>[5x]MLVSVYLALLVACVGQAHSQANLMRLKSDLFNRSPMYPGPTKDDPLTVTLGFTLQDIVKVDSSTNEVDLVYYEQQRWKLNSLMWDPNEYGNITDFRTSAADIWTPDITAYSSTRPVQVLSPQIAVVTHDGSVMFIPAQRLSFMCDPTGVDSEEGVTCAVKFGSWVYSGFEIDLKTDTDQVDLSSYYASSKYEILSATQTRQVQHYSCCPEPYIDVNLVVKFRERRAGNGFFRNLFDENLYFQGHHHHHH

Protein-engineering methods have been exploited to produce a surrogate system for the extracellular neurotransmitter-binding site of a heteromeric human ligand-gated ion channel, the glycine receptor. Acetylcholine-binding protein is a highly conserved ortholog of the pLGIC extracellular ligand-binding domain (ECD) with properties similar to nAChR. Mutations affecting key residues in the orthosteric agonist site at the α1(−)/β(+) interface affect the potency of both activation by glycine and inhibition by strychnine. We therefore set out to generate a high-fidelity surrogate of this α1(−)/β(+) orthosteric binding site using the 2α1:3β stoich­iometry [Fig. 1(a)] by exploiting protein-engineering methods and the thermal stability of acetylcholine-binding protein from Aplysia californica (AcAChBP). Ultimately, the highly stable AcAChBP framework has allowed us to introduce nine amino-acid substitutions that have resulted in a stable surrogate for a heteromeric neurotransmitter site that binds glycine.

A previously published structure of the WT AcAChBP–strychnine complex shows a single molecule occupying four of the five orthosteric sites in the asymmetric unit and one site with two ligands bound. We note also that this alkaloid displays a propensity to dimerize or aggregate at high concentrations. Our structure of the WT AcAChBP–strychnine complex displays a single well ordered strychnine in all five binding sites per asymmetric unit and we confine our comparison to this binding pose. The orientation and the position of the alkaloid in both WT AcAChBP structures is very similar. There is a single direct hydrogen bond between the alkaloid and the protein donated by the protonated tertiary amine to the carbonyl of Trp164. The potential hydrogen-bond acceptors on strychnine, ether and amide O atoms, are placed to interact with solvent and in so doing then form bridges to the protein. Strychnine is a promiscuous ligand that is active against different receptors. Electrophysiological assays indicate that the alkaloid, although the prototypical competitive antagonist of GlyR, also displays the same activity against some nAChR subtypes, with IC50 values that range from 350 nM to around 40 µM. The affinity of strychnine interacting with AcAChBP is consistent with the activity that this ligand displays against the orthologous binding sites presented by nAChRs.Here we show that in addition to small-molecule antibiotics, Streptomyces produce and secrete antibacterial protein complexes that feature a large, degenerate repeat-containing polymorphic toxin protein. A cryo-electron microscopy structure of these particles reveals an extended stalk topped by a ringed crown comprising the toxin repeats scaffolding five lectin-tipped spokes, which led us to name them umbrella particles. Streptomyces coelicolor encodes three umbrella particles with distinct toxin and lectin composition. Each contains an amino-terminal twin arginine translocation (TAT) signal, two sets of four ALF repeats (ALF1–ALF8), two extended coiled-coil domains, and variable C-terminal and toxin domains.

Using single-particle cryo-EM, we obtained a structure of the Umb1 complex at an overall resolution of 4.3 Å. Our maps enabled unambiguous placement of UmbC1 into the Umb1 particle. Although the entirety of the UmbC1 ring was clearly resolved at the centre of the umbrella crown, the density gradually decreased in quality towards the distal portion of its stalk. The C-terminal toxin and HINT domains of UmbC1, which, based on our model, would localize to the tip of the stalk, were therefore also not resolved in our map. Given that our map is derived from >350,000 individual Umb1 particles, we assumed that the UmbA portion of each spoke is effectively an ensemble of the four UmbA proteins in a stoichiometry consistent with their representation in our sample. We therefore elected to model UmbA1 at each spoke position because of the following reasons: UmbA1 is the cognate UmbA for the Umb1 particle; our purification of Umb1 particles on the basis of epitope-tagged UmbA1 ensured that UmbA1 populates at least one spoke in each particle imaged; UmbA1 is typical of Umb1-associated UmbA proteins in that it contains a single lectin domain (unlike UmbA4); and UmbA1 is accommodated well within our maps at each spoke position. The interaction of the UmbA trypsin-like domain with UmbB1 placed the lectin domains of UmbA proteins at the distal ends of the Umb1 spokes. At this location, the domains are readily accessible to ligands, an arrangement compatible with a role in target cell receptor engagement. The structure confirmed that UmbC ALF1 and ALF5 do not bind UmbB1. Notably, it also revealed that ALF6 is not bound by UmbB1, producing a particle with five spokes rather than six.

> MRRRIPSRTPGSGAKQKSWFPRRSLQVLLSAGMLSGLLGTPAALAAEPAPLPANVRADIVGYWETGGAGLKAAAEQALLGGDEAIRKFLADAPSIQHDDNRIDAARMAMTGGSGLRQAAKDAIRLSPAELEKFLLYGYEEPLDDDHKVEIARLINLGGPGVREAGKAALQGTAEERELFLNSGQYTAQQDDNRVDVARLATTGGPNVQAAAKVALRGTPEDMVEFLEVGQFTARNRDQEHATIAELIKQAELAGKQADDARKTAEESSKKAVDASQLAKEAAQKAAEETEAAKDDSQKAAVKAKQAADAARAAADAAQEAIGSANAANRAARRAALAAAQTASAATAAAEAANKAYKAAIAAAGDEGKADEAKEAAKQARAAADAATKSGLAAENAGLASAAAATASTAAKSASSNARAAAGAAEEANQHADAAGVHSNEAALAAAEARRHADAADRAADRSSALAQRAATAAYGARDAANSAAEHANKAADYADESAAHAGDSAAYAATAKRNAQAAQEAAKTATAAVTKANEIFKLARETETANLETRTDAAIERARSMKSASETSITASATTQVEALALNDTATELAKEASRPDIDVQATAAKGRQLAMQAMKLLGPWHQEAAARALSGTDQDVLDYLRTRWKEANHNDIRQQIVDLSTQSPYASVRTAAAEALNGTPEQIEAFHTTGQYTAGSDDMKVDVARLANTGGPGVSQAAKTALADGTGKTLATFLQIGQYGERLSDEKVVTARLAETGSPEVQAAAKIALAGPPELLHEFVTTGQYMAKRKDDLADVHVNQVERLLAEGSLIAAEANEDAWRATEAAATAEGAAADAATAAEKAEASAAQAKQHAADADASADAATRSAADAAASAATARDAADRAAQDATAAENSAAEAAFSAAYARDSASKADDAADRARASALAAGKSADEAEAEAKEAWKTTRALAEKEAEEARRKAAEERKRQQEQAGEPKRVCIPHPTRETMIPIMPCAASPDDSMIMPGPVDPTIRAVVWELAGLNDIKACIDKPLSGNCVMAVVGVTPWGKFKLVSKLGNGLDAVKDARGARRTVACLTGAAHSFPAGTRVLMADGTRRSIEQIEAGDLVTATDPTTGETGARTVTRTIHTPDDRNFTDVALADGSTLTSTTHHPYWSQNDQTWKNAGDLEAGDTLRTPQNTAVVIAATHDWPGLQDAYDLTVDGFHSYYVSTGTTDVLVHNNDNPCPDWVSKAWKKLPKRKSGDPTSGYVFEADGTLVWDSVLTSGRSPLSEDISAFLKGSPDFPNFPGYADVAHHAEAKIAWEMRTKMGKGKKLHIVINTNYVCPKVSSPNSMGCKQAVPAILYEDQTLYVHYPGASDALELKGTAKR;>[5x]MANTSRTRQALMAIAVSVLAAGVTTLGVAHADNGDAVAAAAEMPQAVEDFSYPGAAKIQAETGAILKRGNGHMLMTSCDGSEDIQVMSRTGQKDFCFNVMAKPAYLTLEVPQAYGIWTSADPVKTTIKDTDGTATVINAPANDFTGYGEAGSTGEPTTLIELRVAG;>[5x]MFRMPRPIRATALSAAVLAGALASTPAQATVGDPTTDAKLDFTARLTIGTDYRSCSGALVDTQWVLTAASCFADDPNQPDTVAAGKPAQLTRATVGRADSNIANGYVREVVELVPHPERDMVLARLDKAIPDIAPVRLASDAPTAGTPLTAVGFGRTKDEWVPIQRHQGAFTVTSVTAGAVNVTGQGGDAICAGDTGGPLLQDKNGTLHLVGVNNRSMQGGCYGSETTSTDAIAAMSDADFVTQTVNRDLGTGNLSDLVASADFNSDGRTDVAAVLEDGSLHAFYAKPDGTLEYGRELWNDNTWSPMVQIIGGDFNSDGNGDIAAVRSDGTLNLYTGTATGILNKSKPMWHDTSWKTIKQVTRFKFNGRDGLVAQWGDGNLYGYYTGTDGTLTGTKVKMWPDATWGKTRLTGTADINADGRDDLTAVRDDGSLNWYAGNTKGGLDAARKLWPDNTWTPMKRIIGGDFNGDNKGDIAAVGGQSTLLLYTGTGTGTLNKGIAMRPASGSHHHHHHHH> MAKIGLFFGSNTGKTRKVAKSIKKRFDDETMSDALNVNRVSAEDFAQYQFLILGTPTLGEGELPGLSSDCENESWEEFLPKIEGLDFSGKTVALFGLGDQVGYPENYLDALGELYSFFKDRGAKIVGSWSTDGYEFESSEAVVDGKFVGLALDLDNQSGKTDERVAAWLAQIAPEFGLSL

Azotobacter vinelandii flavodoxin II serves as a physiological reductant of nitrogenase, the enzyme system mediating biological nitrogen fixation. A. vinelandii flavodoxin II is a prototypical long chain flavodoxin with a non‐covalently bound flavin mononucleotide (FMN) cofactor. This cofactor can exist in three different oxidation states: oxidized quinone, one‐electron reduced semiquinone, and two‐electron reduced hydroquinone. When bound by flavodoxin, however, the semiquinone form of FMN is stabilized, which allows for the sequential transfer of one electron at low potentials.

The crystal structure of A. vinelandii flavodoxin II was solved at 1.17 Å resolution by molecular replacement using the model of the Cys69Ala mutant of A. vinelandii flavodoxin II (PDB ID 1YOB19). Following refinement (with statistics presented in Supporting Information Table S2), the root mean square displacements between the wildtype and Cys69Ala variant are 0.45 Å and 0.97 Å based on superpositions of the Cα and all atoms, respectively. No phosphodiester modification was observed in the structure, as has been reported previously to be present in A. vinelandii flavodoxin II;22, 23, 24, 25, 26 perhaps reflecting strain variations or differences in growth conditions. The Azotobacter flavodoxin II also has an insertion of eight amino acid residues (amino acids 64–71) near the FMN cofactor that is generally found in nitrogenase‐associated flavodoxins; these residues have been proposed to be involved in complex formation with the Fe‐protein of nitrogenase. In wildtype flavodoxin II, the Cys69 side chain points toward the interior of the protein near the FMN cofactor, so that formation of a disulfide‐bridged flavodoxin II dimer would require repositioning of this loop. The SG of Cys69 is in van der Waals contact (3.51 Å) with the CD1 methyl group of Leu57, and the presence of this non‐covalent interaction is likely reflected in the variations in the positioning of the FMN and residues 57–60 observed in this region between the wildtype and mutant structures. On reduction to the semiquinone state, the amide bond flips such that the carbonyl is placed in an “O‐up” conformation that is able to hydrogen bond with the protonated N5 position of FMN. The ambiguous electron density for the peptide bond between Gly58‐Glu59, as well as weak density for the side chain of Glu59 in the wildtype flavodoxin II structure [Fig. 3(D)], is indicative of a mixture of conformations that could not be cleanly resolved into components such as cis “O‐down,” trans “O‐down” and trans “O‐up” conformations for a Clostridial flavodoxin. Given the yellow color of the crystals, it is very likely that they exhibit an oxidized state, but the presence of some residual reduced forms from the anaerobic purification and/or photoreduction in the X‐ray beam cannot be dismissed due to weak electron density for Gly58‐Glu59.> SVLQVLHIPDERLRKVAKPVEEVNAEI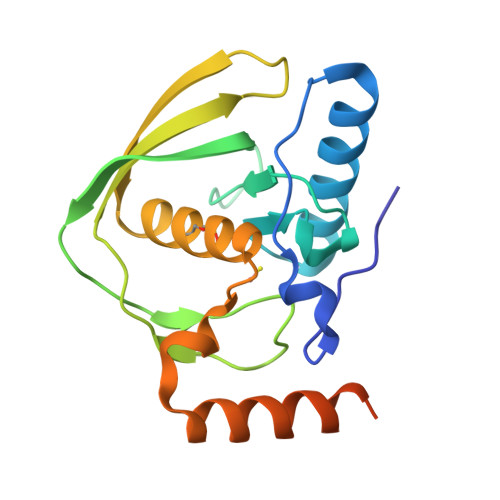QRIVDDMFETMYAEEGIGLAATQVDIHQRIIVIDVSENRDERLVLINPELLEKSGETGIEEGCLSIPEQRALVPRAEKVKIRALDRDGKPFELEADGLLAICIQHEMDHLVGKLFMDYLSPLKQQRIRQKVEKLDRLKARASSSVDKLAAALEHHHHHH Egg-white avidin, similarly to streptavidin from the bacterium Streptomyces avidinii, is a small, tetrameric protein which belongs to the calycin superfamily. The interaction between avidin and biotin, its natural ligand, is one of the strongest non-covalent interactions known in biology (dissociation constant of ~10−15 M) and has been extensively characterized for more than three decades. The structural motif of this protein consists of an eight-stranded antiparallel β-barrel surrounded by flexible loops. In the present work, we have determined the first crystal structures of the avidin complexes with two fluorescent pyrene-biotin conjugates: 1-biotinylpyrene (B9P) and 1-desthiobiotinylpyrene (D9P), which were obtained via a Friedel–Crafts acylation of pyrene with biotin or desthiobiotin, respectively.

Interestingly, initial screens for the second complex (avidin/D9P) produced crystals in several crystallization conditions. The crystals belong to the orthorhombic space group P212121, with the unit-cell parameters a = 57.16, b = 81.95, and c = 107.89 for avidin/B9P and a = 58.97, b = 81.52, and c = 107.78 for avidin/D9P. The final models of the avidin/B9P and avidin/D9P complexes were refined to resolutions of 2.0 Å and 2.1 Å, respectively. The B9P molecule consists of the ureido ring, tetrahydrothiophene ring, valeric acid, and the pyrene moiety, while D9P molecule includes the methyl group and methylene bridge instead of the tetrahydrothiophene ring. The binding cavity in each subunit of avidin is occupied by a single ligand molecule with the same orientation, with the ring system of biotin and desthiobiotin moieties hidden deeply inside the β-barrel, while the pyrene moiety is located at the barrel entrance. In both avidin–pyrene conjugate complexes, well-defined electron density allowed for the determination of the position of B9P and D9P in monomer C, but the pyrene moieties of D9P are not equally well visible in the electron density maps in all monomers that form the avidin tetramer. Photo-degradation of the pyrene ring is most likely observed in two monomers in the avidin/D9P complex, and only part of the ligand was included in the final model. This degradation is more effective for the monomer where the β-barrel opening site is exposed to the solvent channels. For molecules involved in more extensive crystal contacts, less degradation was observed. The sulfur atom from the tetrahydrothiophene ring of B9P acts as an acceptor for the hydroxyl group of Thr77, while in the case of D9P there is no equivalent interaction.

>ARKCSLTGKWTNDLGSNMTIGAVNSRGEFTGTYTTAVTATSNEIKESPLHGTQNTINKRTQPTFGFTVNWKFSESTTVFTGQCFIDRNGKEVLKTMWLLRSSVNDIGDDWKATRVGINIFTRLRTQKE[4x]> MGSSHHHHHHSSGLVPAGSHMAGTKKGVSAAAFSGVTAALGDVGARWFYTWAADPQGITAPAG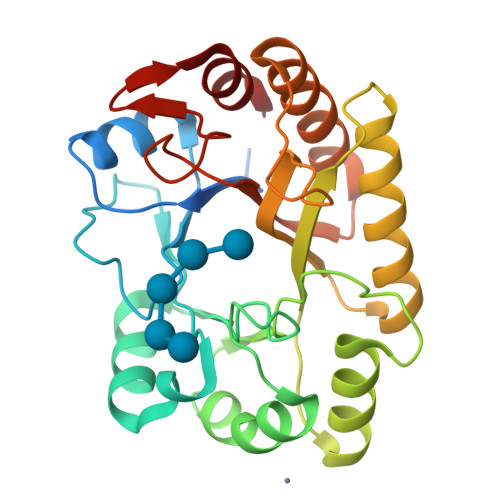TEFVPMIWGRDSVTADQLQRAKAAGSTLLAFNAPDLAGQANMSVETALDLWPQLQATGMRLGAPAVAYGGDTPGGWLDRFMSGAAARGYRVDFIPLHWYGGDFSAAATGQLQSYLQAVYNRYHRPIWLTEYALTDFSGSTPRYPSAAEQADFVSRSTAMLNGLSFVERYAWFSLSTSTTPTGLYTGTTPNSSGVAYRAAG>GAMRIMRPDDANVAGNVHGGTILKMIEEAGAIISTRHCNSQNGERCVAALARVERT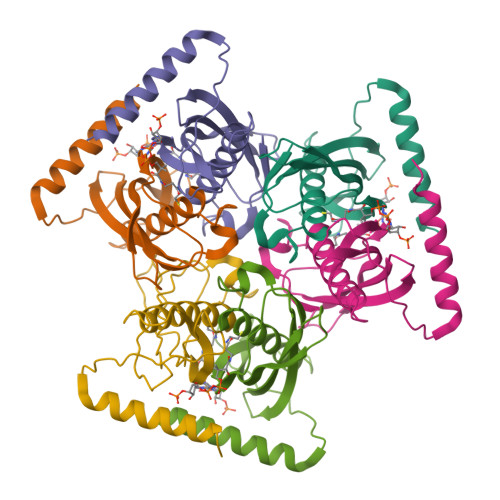DFLSPMCIGEVAHVSAEITYTSKHSVEVQVHVMSENILTGTKKLTNKATLWYVPLSLKNVDKVLEVPPIVYLRQEQEEEGRKRYEAQKLERMETK[6x]> MGHHHHHHHHAIAENLYFQSAAGLHISDGRLVEGNGNDFVMRGINHAHTWYPGETQSLADIKATGANTVRVVLSDGYRWSENSPEDVASIIARCKAERLICVLEVHDTTGYGEDAAAGTLDHAADYWIGLKDVLDGEEDYVVINIGNEPWGNADPAGWTAPTTAAIQKLRAAGFAHTIMVDAPNWGQDWEGVMRADARSVYDADPTGNLIFSIHMYSVYDTAAKVTDYLNAFVDAGLPLLIGEFGGPADQYGDPDEDTMMATAEELGLGYLAWSWSGNTDPVLDLVLDFDPTRLSSWGERVLHGPDGITETSREATVFGGGQGGGDTEAPTAPGTPT

In this study, we report biochemical and structural properties of SACTE_2347, a GH5 mannanase from the cellulolytic SirexAA-E. SACTE_2347 is a member of the GH5 subfamily 8. SACTE_2347 is a three-domain protein that consists of a GH5 catalytic domain (residues 63–308), a fibronectin type-III domain (Fn3, residues 362–437), and a CBM2 (residues 459–559) that are connected by two short linkers (residues 309–361 and residues 438–458). In SACTE_2347, these eight residues correspond to Arg100, His136, Asn177, Glu178, His244, Tyr246, Glu273, and Trp303, with Glu178 and Glu273 serving as the catalytic acid/base and nucleophile, respectively. The conservation of active site residues and the distances between the catalytic acid and base suggests that SACTE_2347 hydrolyzes glycosidic bonds with retention of the anomeric configuration through a double displacement mechanism.

Additionally, we report the atomic resolution (1.06 Å) crystal structure of the GH5 domain of SACTE_2347, which revealed a unique arrangement of two loops adjacent to the active site channel. Crystal of His-tagged SACTE_2347_34kDa belonged to the P21212 space group and contained one monomer per asymmetric unit. The SACTE_2347_32kDa structure has a His tag from a symmetry related monomer bound in the active site channel. Thus, the presence of the bound His tag is not likely to have a significant impact on the position of L1 and L2 in the SACTE_2347_34KDa structure. The SACTE_2347_34kDa and TfManA structures differ substantially in lengths and positions of two loops, L1 and L2, that form part of the active site channel. Interestingly, Tyr281 from SACTE_2347_34kDa is positioned at the tip of L1, where it could interact with a bound mannan chain sugar, but also provide steric exclusion to the placement of an α-1, 6 linkaged glucomannan unit into the +1 and perhaps the +2 subsites. Furthermore, L2 loop (residues 302–315) in the SACTE_2347_34kDa is two residues shorter and shifted toward the −3 site as compared to L2 loop of TfManA. Furthermore, L1 and L2 do not make contacts with each other in SACTE_2347_34kDa, but instead provide an opening between the two loops that is perpendicular to the main path of the channel and above the catalytic residues. The space between L1 and L2 is large enough to allow a branching sugar to bind in the −1 position.>[2x]MKKIFMMVHELDVNKGGMTSSMFNRSKEFYDADIPADIVTFDYKGNYDEIIKALKKQGKMDRRTKMYNVFEYFKQISNNKHFKSNKLLYKHISERLKNTIEIEESKGISRYFDITTRTYIAYIRKSKSEKVIDFFKDNKRIERFSFIDNKVHMKETFNVDNKVCYQVFYDEKGYPYISRNINANNGAVGKTYVLVNKKEFKNNLAL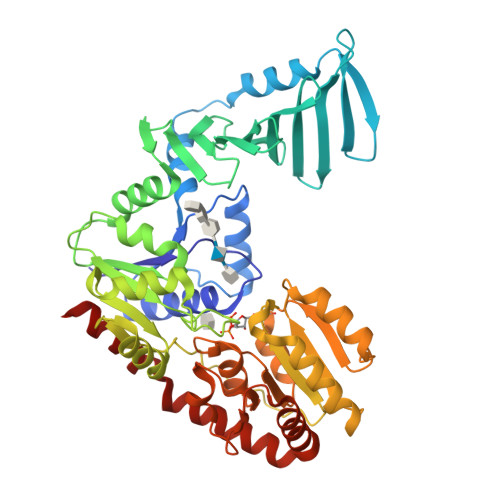CVYYLEKLIKDSKDSIMICDGPGSFPKMFNTNHKNAQKYGVIHVNHHENFDDTGAFKKSEKYIIENANKINGVIVLTEAQRLDILNQFDVENIFTISNFVKIHNAPKHFQTEKIVGHISRMVPTKRIDLLIEVAELVVKKDNAVKFHIYGEGSVKDKIAKMIEDKNLERNVFLKGYTTTPQKCLEDFKLVVSTSQYEGQGLSMIEAMISKRPVVAFDIKYGPSDFIEDNKNGYLIENHNINDMADKILQLVNNDVLAAEFGSKARENIIEKYSTESILEKWLNLFNS> HGTELPSPPSVWFEAEFFHHILHWTPIPQQSESTCYEVALLRYGIESWNSISQCSQTLSYDLTAVTLDLYHSNGYRARVRAVDGSRHSQWTVTNTRFSVDEVTLTVGSVNLEIHNGFILGKIQLPRPKMAPAQDTYESIFSHFREYEIAIRKVPGQFTFTHKKVKHEQFSLLTSGEVGEFCVQVKPSVASRSNKGMW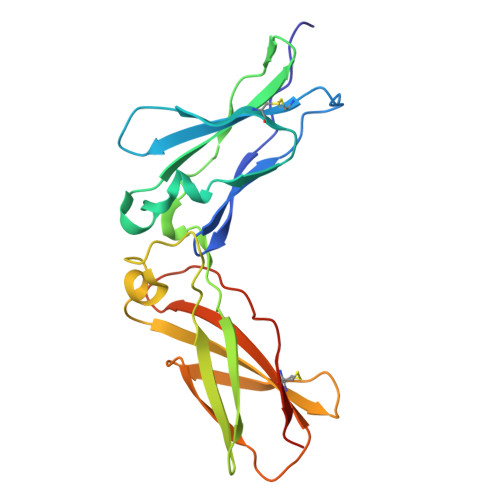SKEECISLTRQYFTVTN> MLPLAALNMRVRRRLSLFLNVRTQVAADWTALAEEMDFEYLEIRQLETQADPTGRLLDAWQGRPGASVGRLL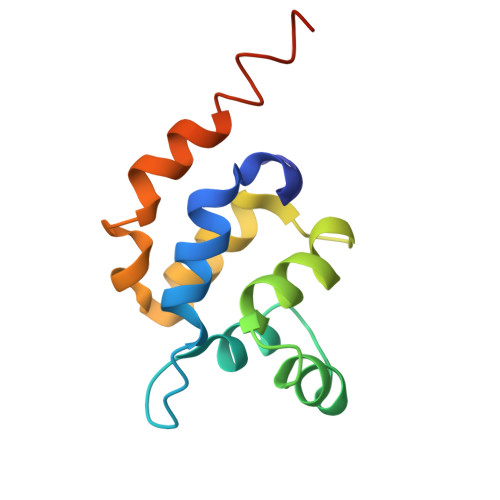ELLTKLGRDDVLLELGPSIEEDCQKYIAAALEHHHHHH> MSCTTRRFIDEKEKLEYSRGYNQQELEASKLRKDFVKKYIVDFDTTLYKTQVERDWAYIAKREYRYEVQLKSIGYGG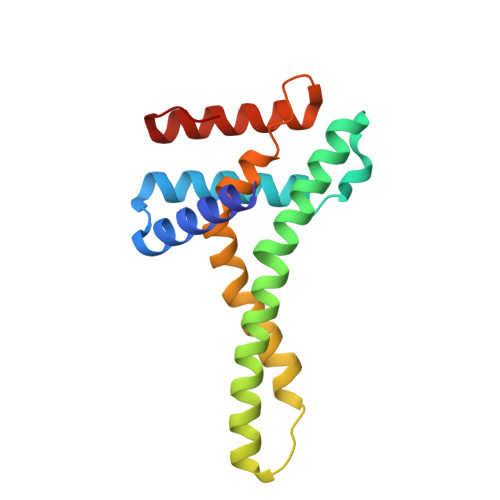ALANAVLLWRIYANKKMVFWPIPIVGALGYLYFQPVFFQKSNKRFFDMCNVGEEYYLGRERNKILRECNKILNVEDF Carrageenans, alongside agars, are the main cell wall polysaccharides of red macroalgae and play vital roles in the development and physiology of these photosynthetic eukaryotes. In marine ecosystems carrageenans constitute a huge biomass and thus a precious carbon source for marine heterotrophic bacteria (MHB). The marine Bacteroidetes Zobellia galactanivorans DsijT, originally isolated from a healthy red macroalga, is a bacterial model for the bioconversion of algal polysaccharides. Here we describe in Z. galactanivorans the discovery and the integrative characterization of the complete pathway for utilization of the kappa family carrageenans (containing 3,6-anhydro-d-galactose units, mainly kappa-, iota- and beta-carrageenans), which is carried out by a complex regulon including a dedicated atypical PUL, lacking the susCD-like pair, and carrageenan-induced loner genes including distal susCD-like pairs.

Thus, these enzymes are exo-lytic α-1,3-(3,6-anhydro)-d-galactosidases which cleave the α-1,3 linkage between D-AnG and d-galactose on the non-reducing end, releasing D-AnG and odd-DP (degree of polymerization) oligocarrageenans. ZGAL_3152 forms a homodimer and the monomer has a complex architecture with an N-terminal distorted beta-sandwich domain (Pro35-Asp299), a central TIM barrel (Tyr300-Lys620) and a C-terminal immunoglobulin-like domain (Glu621-Asp693). The dimeric interface is mainly formed by the interaction of long loops from the TIM-barrel (342–357 and 430–459) with the two helices protruding from the N-terminal domain (η3 and α2) of the other monomer. The dimer is also stabilized by the swapping of the C-terminal strand β36. There are two predicted active sites at either side of the base of an impressive crevasse that is 60 Å long and 40 Å deep. Numerous trials for obtaining the structure of ZGAL_3152 complexes were performed, but they were unsuccessful; however, buffer molecules found in the active site of each ZGAL_3152 monomer likely mimic monosaccharide units. In chain C, a Tris, an MDP and a second Tris are bound in the potential subsites −1, +1, and +2, respectively. The residues interacting with these buffer molecules (Cys198, Lys208, Asn218, His347, Trp455, Leu536, and Gln566) are well conserved in ZGAL_3152 homologs, suggesting their implication in substrate recognition. Three are located in one monomer from the homodimer (Asp486, Glu517, and Glu531), while Asp202 originates from helix α2 of the second monomer. Asp202, Asp486, and Glu517 are strictly conserved. Site-directed mutagenesis of the four candidates yielded soluble inactive enzymes; these residues are thus involved in the catalytic machinery, although the structure of a substrate-enzyme complex would be needed to determine their respective roles.

>[4x]MKNNSTVAKSTLVLLVVTCLTAFKGLAFDSISPDPIVLENGKLNINIDSKTGCFSVTEKTSGHVWKSDPWENAAGLLTLTDSKGKKQTVNISKSKKIEVSKTAKNTVSLKFIDPVFEDGSVAKGVSIATELRLDPNNAQLDVEVTEHRSGNFTLYDLRYPARAFSLKTDEDKGAAVIPQKQGVICPSYIFPMNGGRFCKWDDATYNNKSQGSLELFNNGTGLTMPWWGTYNEKSAVMGIVDVSARPHMQYNINNNGQYLFNAKGVMSPYQRIVFLDPIWKLDQEKGKMRISYHFIPGGDYVDMAKVYQKEAKARGHFVSLQEKLKRNPNVNKLPGAIYFGIYGGYPHYVNMPGMAFTFDELKNIIKTIHDDLRVDKAFVHAWGTFSNFVPHNYPISEALGGPEKLKAAVDLAKSYGYLYSSYHAYSPMLENDPNFTTDLMQRDAEGKLMNTGSRWARVDPKFQKGLAQKNIEKEISYLGLEADITDITFAAYRENGKEGRIELAKYIDSFNLVNGTEHGQEQWIPYFDMFEGMTYLEDRPLSVISHPAPLFNLVYHEAIANFGKIQDPDNEVTANGDFRIKALRSMLFGRGTTIFFAPYEFEGMRPMIEMARDLVSPVHKETFYSELKSHEYLSADYKVQRSRFSSGTEVIANLGPVAQKIEGGISIPGYGYRIQMKDGSLKTGHFQVSLHMD SPIRONOLACTONE | 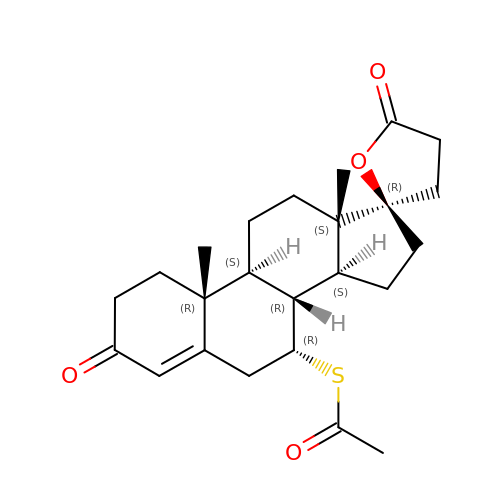C24 H32 O4 S | LXMSZDCAJNLERA-ZHYRCANASA-N7-fluoranyl-5-(4-methylphenyl)sulfonyl-quinolin-8-ol 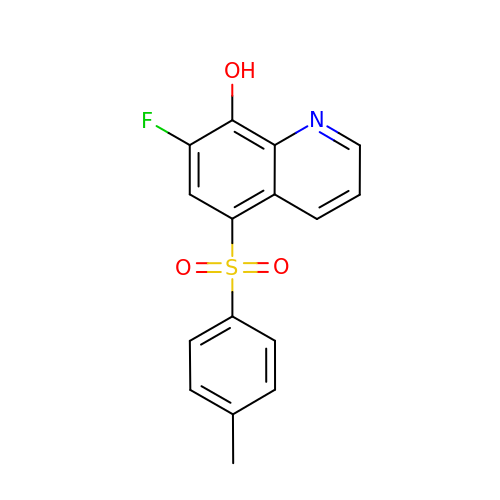| C16 H12 F N O3 S | VRULDRRQTAPONR-UHFFFAOYSA-N> GQQKQKMNSKH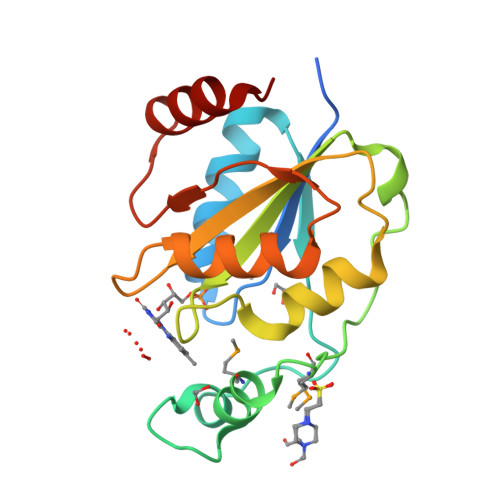SNSKILVAYFSATGTTARAAEKLGAAVGGDLYPIAPAQPYTSADLDWNNKRSRSSVEMNDPKMRPAIKSKKENIGTYDVVFIGYPIWWDLAPRIINTFIEGHSLKGKTVVPFATSGGSSIGNSATVLKKTYPDLNWKEGRLLNRTDEKAIRAWLDVIAVK> GSHMIARIIGEIGIEGARFIEENIDEQFKALRYLSKGIDSETFVKLVIANSLVSYQLTGKGEQWWWEFAKYFYGRDVKSIYLAYKEFLPNSRFNRRLIPQKLSRIRRVETFLSTLTEERIEEYYGDMSSLWGSIARALGVDKESQTVVFSVKMFGYAARIVLSTFNPYPMEIPIPEDSRIVKLTKKLTNEKPRKFWMKIARESGVPPLHIDSILWPLLGGASIDSAPPELRDKLAELIKIIR

8-Oxoguanine (GO) is a major purine oxidation product in DNA. The major way to remove GO is the base excision repair pathway, usually initiated by a GO-DNA glycosylase. While no enzymes with an A/G specific-DNA glycosylase or a dGOTPase activity have been discovered in these species, a GO-DNA glycosylase called AGOG (for Archaeal GO-DNA Glycosylase) has been initially identified in the hyperthermophilic archaeon Pyrobaculum aerophilum. Despite very low sequence identity, AGOG is structurally similar to eukaryotic and prokaryotic OGG1 and OGG2 GO-DNA glycosylases and, like these two proteins, belongs to the Endo III structural superfamily partly defined by the central helix-hairpin-helix (HhH) element followed by a glycine/proline-rich region and an aspartate (GPD).

To clarify the mode of recognition of GO in double-stranded DNA prior to the cleavage of its N-glycosidic bond by AGOG, we solved the 3D structure of a mutated K142Q-Pab-AGOG, a catalytically defective mutant which has kept its substrate recognition ability, complexed with a GO-containing 9-mer DNA duplex at 1.25 Å resolution (Pab-AGOG/dsDNA-GO:C). In this structure, the protein interacts with the estranged C in the same way as observed for the borohydride-trapped AP lesion with an opposite C while the GO nucleotide is extruded from the DNA helix and stabilized inside the enzyme active site in an anti-conformation similar to that previously observed for the OGG1 and OGG2 enzymes. The space in the DNA double-helix vacated by the flipped GO is partially filled by Q53 and R93 as seen in the crystal structures of the trapped Pab-AGOG-dsDNA-C. First, the O8 atom of the GO-containing DNA is no longer contacted by W62 and second, the ribose moiety is flipped and makes an H-bond with D174. This leads to the repositioning of the sidechain of Q142 (K in wild type) towards the GO-sugar moiety. Similarly to OGG1 and OGG2, Pab-AGOG does not interact with the 8-oxo-carbonyl of GO but recognizes the N7-H of GO by a strictly conserved glutamine residue (Q24). In the Pab-AGOG/dsDNA-GOC structure, the GO lesion is not the only base extruded from the DNA helix. In fact, the thymine upstream of the lesion (T3) is not paired with A7* as expected but rather stacks on the G56 residue of a well-conserved loop between the α4 and α5 helices. Moreover, R176 stabilizes the phosphate group between the two extruded bases (GO and T3), which contrasts with what we observed in the structure Pab-AGOG complexed to the AP site, where no contact between R176 and DNA was present. However, the double base flipping on the damaged strand has never been observed for any DNA glycosylases.> YQYKDILSVFEDAFVDNFDCKDVQDMPKSILSKEEIDHIIMSKDAVSGTLRLFWTLLSKQEEMVQKFVEEVLRINYKFLMSPIKTEQRQPSMMTRMYIEQRDRLYNDNQVFAKYNVSRLQPYLKL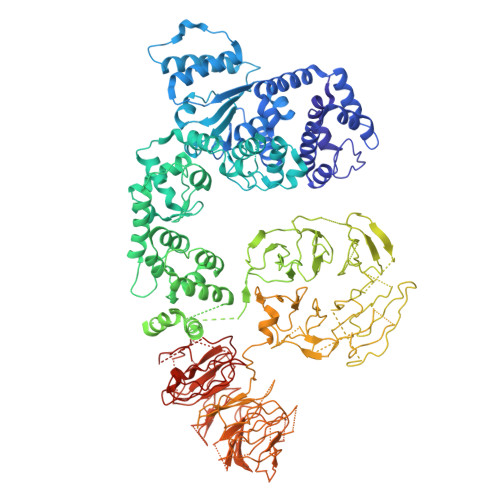RQALLELRPAKNVLIDGVLGSGKTWVALDVCLSYKVQCKMDFKIFWLNLKNCNSPETVLEMLQKLLYQIDPNWTSRSDHSSNIKLRIHSIQAELRRLLKSKPYENCLLVLLNVQNAKAWNAFNLSCKILLTTRFKQVTDFLSAATTTHISLDHHSMTLTPDEVKSLLLKYLDCRPQDLPREVLTTNPRRLSIIAESIRDGLATWDNWKHVNCDKLTTIIESSLNVLEPAEYRKMFDRLSVFPPSAHIPTILLSLIWFDVIKSDVMVVVNKLHKYSLVEKQPKESTISIPSIYLELKVKLENEYALHRSIVDHYNIPKTFDSDDLIPPYLDQYFYSHIGHHLKNIEHPERMTLFRMVFLDFRFLEQKIRHDSTAWNASGSILNTLQQLKFYKPYICDNDPKYERLVNAILDFLPKIEENLICSKYTDLLRIALMAEDEAIFEEAHKQVQRFDDRVWFTNHGRFHQHRQIINLGDNEGRHAVYLHNDFCLIALASGQILLTDVSLEGEDTYLLRDESDSSDILRMAVFNQQKHLITLHCNGSVKLWSLWPDCPGRRHSGGSKQQLVNSVVKRFIGSYANLKIVAFYLNEDAGLPEANIQLHVAFINGDVSILNWDEQDQEFKLSHVPVLKTMQSGIRCFVQVLKRYYVVCTSNCTLTVWDLTNGSSNTLELHVFNVENDTPLALDVFDERSKTATVLLIFKYSVWRLNFLPGLSVSLQSEAVQLPEGSFITCGKRSTDGRYLLLGTSEGLIVYDLKISDPVLRSNVSEHIECVDIYELFDPVYKYIVLCGAKGKQVVHVHTLRSVSGSNSHQNREIAWVHSADEISVMTKACLEPNVYLRSLMDMTRERTQLLAVDSKERIHLIKPAISRISEWSTITPTHAASNCKINAISAFNDEQIFVGYVDGVIIDVIHDTALPQQFIEEPIDYLKQVSPNILVASAHSAQKTVIFQLEKIDPLQPNDQWPLMMDVSTKYASLQEGQYIILFSDHGVCHLDIANPSAFVKPKDSEEYIVGFDLKNSLLFLAYENNIIDVFRLIFSCNQLRYEQICEEEIAQKAKISYLVATDDGTMLAMGFENGTLELFAVENRKVQLIYSIEEVHEHCIRQLLFSPCKL>MAHHHHHHAMQFDVTIEIPKGQRNKYEVDHETGRVRLDRYLYTPMAYPTDYGFIEDTLGDDGDPLDALVLLPQPVFPGVLVAARPVGMFRMVDEHGGDD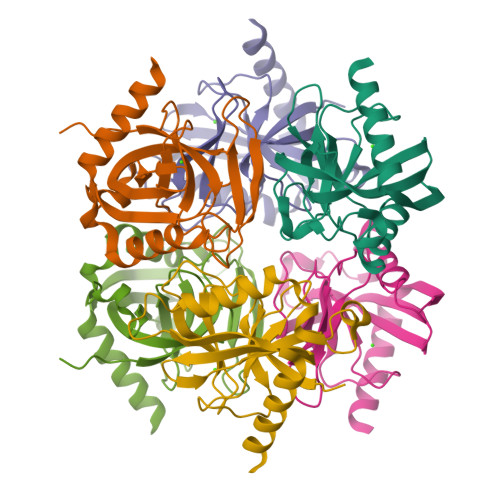KVLCVPAGDPRWDHVQDIGDVPAFELDAIKHFFVHYKDLEPGKFVKAADWVDRAEAEAEVQRSVERFKAGTH[3x]2-(2,2-diphosphonoethyl)-1-methylpyridin-1-ium 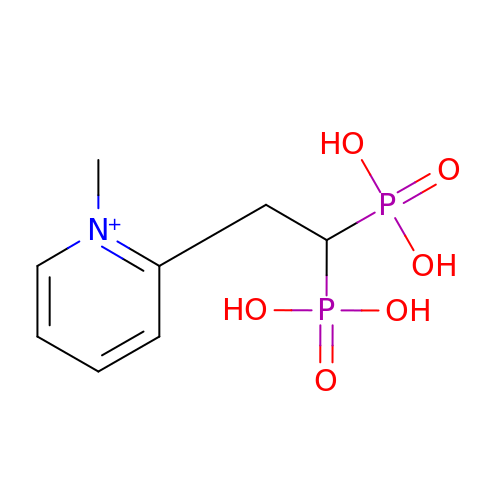| C8 H14 N O6 P2 | DNSXFQJOCNECTD-UHFFFAOYSA-O Here, we present the near-atomic resolution structure of Haloferax tailed virus 1 (HFTV1), an archaeal virus thriving in extreme salinity. Through single-particle analysis, we obtained near-atomic resolution maps of DNA-filled and empty virions, enabling us to assemble full atomic models of the virus pre- and post-DNA release, including all structural protein components. The full atomic structure revealed that the virus has a length of 1350 Å and an icosahedral head with a diameter of ~600 Å. The tail has a length of 560 Å and terminates into a baseplate with three radiating TFs of ~190 Å in length.

The final TTP hexamer is followed by the trimeric BTC, which in turn interfaces with the trimeric BPH. Notably, the BTC protein is a pseudo-hexameric trimer: Each subunit consists of two homologous domains, which have likely arisen through a gene duplication and fusion event. The BPH coordinates Mg2+ and K+ ions that likely contribute to the stability of the complex, and connects to the BTC via a triangular ring, from which three globular domains project. Curiously, these domains show an asymmetric configuration. While two of the domains are bound to each other, one remains unbound. As the binding interfaces of these three domains are equal, it can be assumed that they are free to interchange. This suggests that the three BPH domains may undergo dynamic cycles of binding and unbinding, which in turn may aid virus’ docking or penetration of the S-layer. Specifically, the three folded-back TMP termini interact with the trimeric baseplate-tail connector (BTC; gp41), while the three extended termini engage the trimeric BPH protein. The BPH also anchors three TFs. The C-terminal end of the BPH contains a predicted carbohydrate/galactose-binding domain, which may interact with remaining glycan residues on the S-layer or lipid-glycan carriers embedded in the membrane.

>[6x]MATSPEGIWSNSGALTFEDPADDSEILFAGVRDVTITPAYEHAELYTIDSTFRDEVKRYEHNVNVEITYAKFSLEFAQEWLGGPGATATASQDDSDPMKFNLENVTPSASGGFERTTAVENVVFPELPLDSATYGEYEEYSLTGSGRSVTNLADTSGV;>[3x]MVDATLSRGGTSVDIPLVEEGGEILLSSTFGKPEVNVRKSGGSLNPRVIDSWSGLQTFQLVGKLYDYSTSHQLADLVKTASTTPLELQIPQDAYPDTVTVAPAAGQASALTLEYPAGRKDLVDVSLSLTRVDPNSVRGVGDQQATTPTTTGTGPVEVTAGGTTVQLPSSGLSVERTVGRPNDAVRRVPRQADPRYEVKAKVTNDVFTFSFETLDNIPATLNALTDNVFREQLGRDGVTLDFNGLLGLGSVKAIPVGSSPFRQVHQAGRGWVTVPTLEFRRIYSNE;>MPQLGDSKLGESQLGSPGTLKQGVEWTVVVDGEEQNNVWDVQVVDTANPFGDYAVFKMDDRGGQAFEAYPRGTRVEAYVSEGTEPLDNRFTGYVVERRENEQQGADVLEVEAYSFDQFLRRNTVTNDQTGNTISQALADIIQTDTPVRFNAANITVGDDQELTRSYQGDPVENALRDFAFKSTNEDFGVGDDLEFFFQPRETVHIDRGVDNTQWFRYDIPELGKEAINEVEVWFDDGEESVIVDDGTDKLDLQDSLGLPSPGTQRKELQRPLVTDISDAEDIGRKYLAFRNSTLSGTVTTYGLYDAEPGDTIDITIDPRGIDEEFVIAAIEYRWGVDETILTVVEKRGDVDDILSELSESVQRIEMQGANRDAPKNRITTTNAAAIVSVDVDAGGTSADADRFVNDGRNAVRDAWTGAGNPDIANIVVGDDNSGLSRTNTTLGNQTDSVSVTESLPSAKVVEYSATLTQSGVEEIGLETSTGTLLTRATFETPVDLSSDTVTVTLTVSNDDSVSRGVMTNDGQTAVRDVLADNSPTLPTDYGYGDDSTAVAETDTTLGNELANTSLEEILIQSASSVSAWNTILGTLASTYPLVVSSSGIRPAQTAWTTESDNLAQSGTALVTVGDYSNGEAEGLDSPGDTLELSFTPEHDIPGEEFALWCRIETDLGGTDPGPEITVTLDIDGDTYSWVPIGTNTALGLNWYDLANNTFGGSSTYPDTDIPEGSTVTLSIEATSSSVSGQGHAVDVMAPLDALTRVTGGSDATSAYTFDNNNGGSGGYLDGPELYPDQLILSLETATTRRNVSEARFTLTANDTSGNFYVELANDGSTFNRVNNATSGSVTFASPDTNVDTNISLNRYGSRSTATPQTGFNAQEIDNWELYADIDAVLPDDIGVTLSRAIIPPNTSGIVGQTVREAGLKSGSTLLTRHILAEFLLDTDQRLASSESTRFTSDN[3x];>[9x]MADTTIIDAVVFPQDDGTGVSNGDEDYDSAGYLASLARYAGDGSYVGGDSTGSPTLQFANIDTANEEVDIQPGHAFILESGHIVQSGSQKTYDTNLPDSVPYVVILPSSVTNVPLDTDVDNDVWLAVDPTSNDSVYIRSGNGLSAPSDPSVKLGTVNSSTGSTTRPNDLADHSVDALNATTIDASDTVTGDTVDATTTLTDAAGVSHTGELEDINHGSKHEDGGSDEISVGGLSGDLADPQDPKAHAASHSADSADEISVENLSTTGSADTVPISQGDGTLSMGS;>MVAIRSEGVSETQQNLEGVENAMEDTADSAGDSAAELETFSKRFKGAMGAAVSALAIGTAGLLSQVPVVGEAMGGLGAIIDALTMKIDEDARPAVGSFTDDLYEVAEATYEADSSLEAFQTALDGVNTAIDDVAVSTLQTEIEELTGITIPKNWLDFGWDIMTLDARQTMDNIETIINEFPEDFGTMLKSIDPRAKKGWDILTKSADMFINDLTSRIDSGVNDVRGFFTGLASDLNEWGGNVASDAREWGTNLIDKFTGGIRSKISGLRNWLSELRNIGAEVGIDVPTIGGGGDGGGGGGNSSRQPFAGGFFGGGNATIDGRQISESTGRYRSDPSRRRGI[6x]>[2x]QTIQPGTGYNNGYFYSYWNDGHGGVTYTNGPGGQ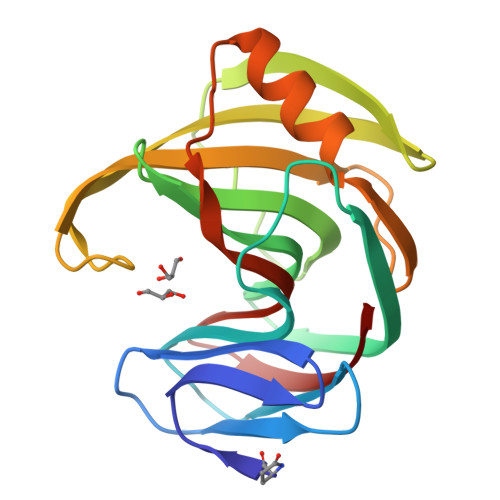FSVNWSNSGNFVGGKGWQPGTKNKVINFSGSYNPNGNSYLSVYGWSRNPLIEYYIVENFGTYNPSTGATKLGEVTSDGSVYDIYRTQRVNQPSIIGTATFYQYWSVRRNHRSSGSVNTANHFNAWAQQGLTLGTMDYQIVAVEGYFSSGSASITVS> WSHPQFEKVPIKYLPEENVHDADFGEQKDISEINLAAGLDLFQGDILLQKSRNGLRDPNTRWTFPIPYILADNLGLNAKGAILYAFEMFRLKSCVDFKPYEGESSYIIFQQFDGCWSEVGDQHVGQNISIGQGCAYKAIIEHEILHALGFYHEQSRTDRDDYVNIWWDQILSGYQHNFDTYDDSLITDLNTPYDYESLMHYQPFSFNKNASVPTITAKIPEFNSII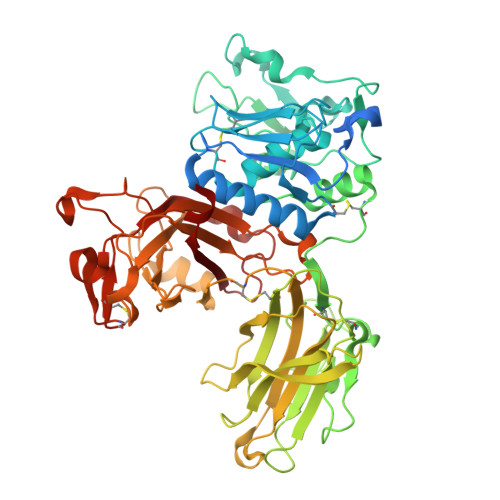GQRLDFSAIDLERLNRMYNCTTTHTLLDHCTFEKANICGMIQGTRDDTDWAHQDSAQAGEVDHTLLGQCTGAGYFMQFSTSSGSAEEAALLESRILYPKRKQQCLQFFYKMTGSPSDRLVVWVRRDDSTGNVRKLVKVQTFQGDDDHNWKIAHVVLKEEQKFRYLFQGTKGDPQNSTGGIYLDDITLTETPCPTGVWTVRNFSQVLENTSKGDKLQSPRFYNSEGYGFGVTLYPNSRESSGYLRLAFHVCSGENDAILEWPVENRQVIITILDQEPDVRNRMSSSMVFTTSKSHTSPAINDTVIWDRPSRVGTYHTDCNCFRSIDLGWSGFISHQMLKRRSFLKNDDLIIFVDFEDITHLS>MRLSYEALEWRTPIENSTEPVSLPPPPPFFGQERAREALELAIRGGFHAYLVGPPSLGKHEALLAYLSTQSVETPPDLLYVPLSERKVAVLTLPSGQEIHLAEAVEGLLLEVNRLDELFRQGSFLREKTQLEARFKEAREQQLEALRREAQEAGFALSTNGERLELTGPGPVPAELSARLEEVTLGSLAASAELEVALRRLRRDWALHYLNNRFEPLFQRFPQARAYLEALRARLARYAETGEPLDPAQWRPNLLTSSSSGTPPPIVYEPYATAPRLFGRLDYLVDRGVWSTNVSLIRPGAVHRAQGGYLILDALSLKREGTWEAFKRALRNGQVEPVTEPQAPAGLEVEPFPIQMQVILVGTPEAFEGLEEDPAFSELFRIRAEFSPTLPASPENCTALGGWLLAQGFQLTQGGLTRLYDEARRMAEQRDRMDARLVEIRALAEEAAVLGGGLLTAESVEQAIAAREHRSFLSEEEFLRAVQEGVIRLRTTGRAVGEVNSLVVVEAAPYWGRPARLTARAAPGRDHLISIDREAGLGGQIFHKAVLTLAGYLRSRYIEHGSLPVTISLAFEQNYVSIEGDSAGLAELVAALSAIGNLPLRQDLAVTGAVDQTGKVLA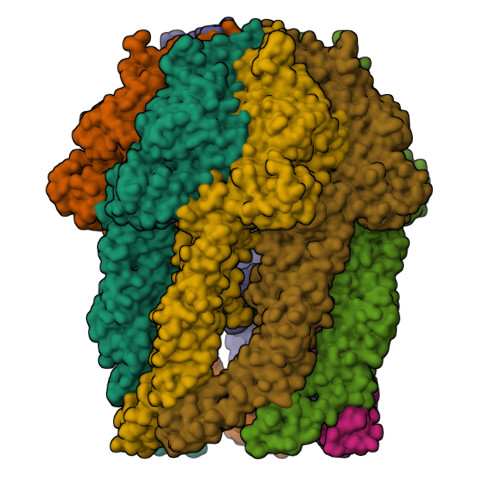VGAINAKVEGFFRVCKALGLSGTQGVILPEANLANLTLRAEVLEAVRAGQFHIYAVETAEQALEILAGARMEGFRGLQEKIRAGLEAFARLEEGHDKEDREKLAAALEHHHHHH[7x]> MIKLGIVMDPIANINIKKDSSFAMLLEAQRRGYELHYMEMGDLYLINGEARAHTRTLNVKQNYEEWFSFVGEQDLPLADLDVILMRKDPPFDTEFIYATYILERAEEKGTLIVNKPQSLRDCNEKLFTAWFSDLTPETLVTRNKAQLKAFWEKHSDIILKPLDGMGGASIFRVKEGDPNLGVIAETLTEHGTRYCMAQNYLPAIKDGDKRVLVVDGEPVPYCLARGGGGEPRPLTESDWKIARQIGPTLKEKGLIFVGLDIIGDRLTEINVTSPTCIREIEAEFPVSITGMLMDAIEARLQQ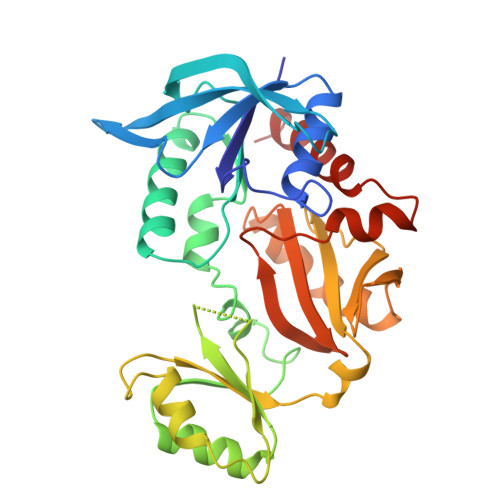Q N~2~-(1-cyclopentyl-4-oxo-4,7-dihydro-1H-pyrazolo[3,4-d]pyrimidin-6-yl)-N-(4-methoxyphenyl)-D-alaninamide 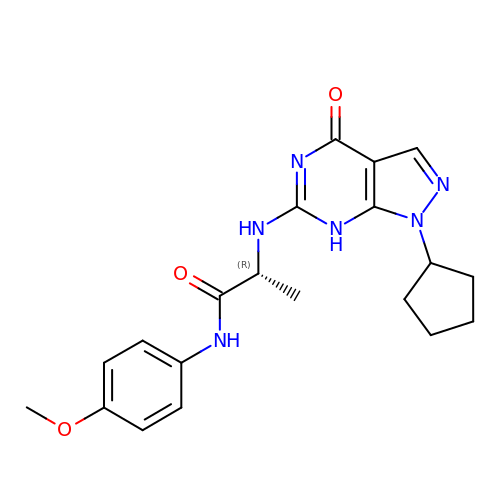| C20 H24 N6 O3 | UBBCZBKJYNXHGT-GFCCVEGCSA-N> EHAERLPYDASKWEFPRDRLKLGKPLGRGAFGQVIEADAFGIDKTATCRTVAVKMLKEGATHSEHRALMSELKILIHIGHHLNVVNLLGACTKPGGPLMVITEFCKFGNLSTYLRSKRNEFVPYKVAPEDLYKDFLTLEHLICYSFQVAKGMEFLASRKCIHRDLAARNILLSEKNVVKICDFGLARDIYKDPDYVRKGDARLPLKWMAPETIFDRVYTIQSDVWSFGVLLWEIFSLGASPYPG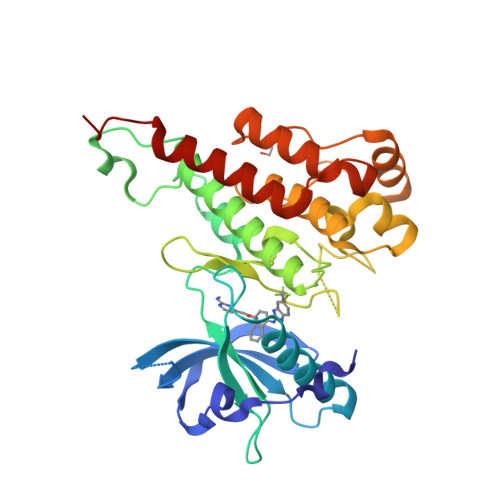VKIDEEFCRRLKEGTRMRAPDYTTPEMYQTMLDCWHGEPSQRPTFSELVEHLGNLLQANAQQDRHHHHHH> MEYEWKPDEQGLQQILQLLKESQSPDTTIQRTVQQKLEQLNQYPDFNNYLIFVLTKLKSEDEPTRSLSGLILKNNVKAHFQNFPNGVTDFIKSECLNNIGDSSPLIRATVGILITTIASKGELQNWPDLLPKLCSLLDSEDYNTCEGAFGALQKICEDSAEILDSDVLDRPLNIMIPKFLQFFKHSSPKIRSHAVACVNQFIISRTQALMLHIDSFIENLFALAGDEEPEVRKNVCRALVMLLEVRMDRLLPHMHNIVEYMLQRTQDQDENVALEACEFWLTLAEQPICKDVLVRHLPKLIPVLVNGMKYSDIDIILLKGDVEGGSGGDDTISDWNLRKCSAAALDVLANVYRDELLPHILPLLKELLFHHEWVVKESGILVLGAIAEGCMQGMIPYLPELIPHLIQCLSDKKALVRSITCWTLSRYAHWVVSQPPDTYLKPLMTELLKRILDSNKRVQEAACSAFATLEEEACTELVP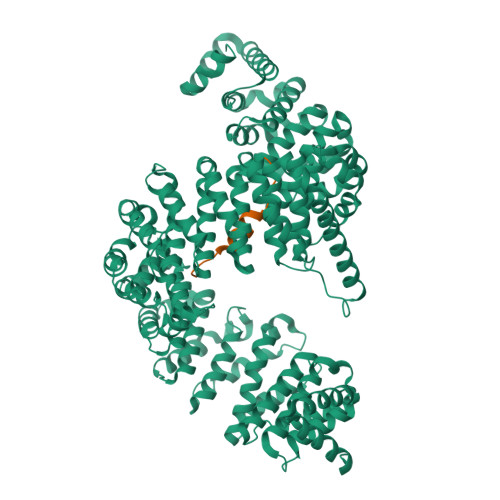YLAYILDTLVFAFSKYQHKNLLILYDAIGTLADSVGHHLNKPEYIQMLMPPLIQKWNMLKDEDKDLFPLLECLSSVATALQSGFLPYCEPVYQRCVNLVQKTLAQAMLNNAQPDQYEAPDKDFMIVALDLLSGLAEGLGGNIEQLVARSNILTLMYQCMQDKMPEVRQSSFALLGDLTKACFQHVKPCIADFMPILGTNLNPEFISVCNNATWAIGEISIQMGIEMQPYIPMVLHQLVEIINRPNTPKTLLENTAITIGRLGYVCPQEVAPMLQQFIRPWCTSLRNIRDNEEKDSAFRGICTMISVNPSGVIQDFIFFCDAVASWINPKDDLRDMFCKILHGFKNQVGDENWRRFSDQFPLPLKERLAAFYGV;> RGGGDRGGFGPGKMDSRGEHRQDRRERPY>[2x]MEAVVVEREAKGM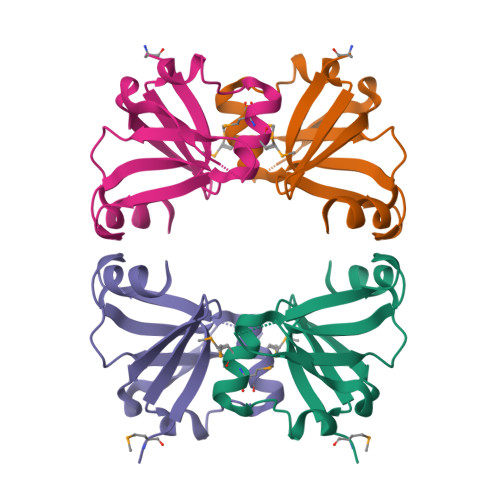KEIAIQEKDLTLQWRGNTGKLVKVRLKNTRAMEMWYNKQITEENIQEITTLNIIKNGKSLALEVYPEKSIYVKPNLGRINVPVFFIKTPINRGVFEEIFGETLKA>MDIWYGTAAVPKDLDNSAVTIGVFDGVHRGHQKLINATVEKAREVGAKAIMVTFDPHPVSVFLPRRAPLGITTLAERFALAESFGIDGVLVIDFTRELSGTSPEKYVEFLLEDTLHASHVVVGANFTFGENAAGTADSLRQICQSRLTVDVIDLLDDEGVRISSTTV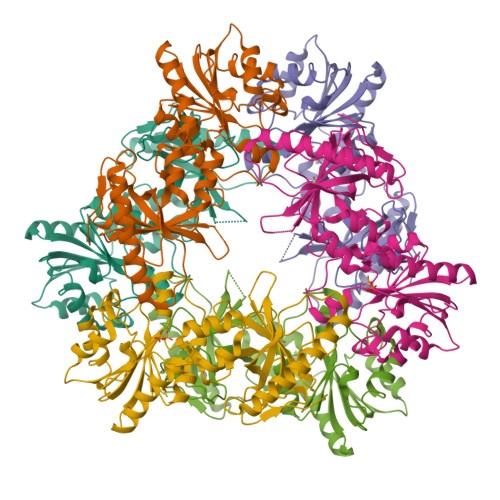REFLSEGDVARANWALGRHFYVTGPVVRGAGRGGKELGWPTANQYFHDTVALPADGVYAGWLTILPTEAPVSGNMEPEVAYAAAISVGTNPTFGDEQRSVESFVLDRDADLYGHDVKVEFVDHVRAMEKFDSVEQLLEVMAKDVQKTRTLLAQDVQAHKMAPETYFLQAES[2x]> MASWSHPQFEKGASTSLYKKAGLMDSQRSTLVHWFRKGLRLHDNPALSHIFTAANAAPGRYFVRPIFILDPGILDWMQVGANRWRFLQQTLEDLDNQLRKLNSRLFVVRGKPAEVFPRIFKSWRVEMLTFETDIEPYSVTRDAAVQKLAKAEGVRVETHCSHTIYNPELVIAKNLGKAPITYQKFLGIVEQLKVPKVLGVPEKLKNMPTPPKDEVEQKDSAAYDCPTMKQLVKRPEELGPNKFPGGETEALRRMEESLKDEIWVARFEKPNTAPNSLEPSTTVLSPYLKFGCLSARLFNQKLKEIIKRQPKHSQPPVSLIGQLMWREFYYTVAAAEPNFDRMLGNVYCMQIPWQEHPDHLEAWTHGRTGYPFIDAIMRQLRQEGWIHHLARMAVACFLTRGDLWISWEEGQRVFEQLLLDQDWALNAGNWMWLSASAFFHQYFRVYSPVAFGKKTDPQGHYIRKYVPE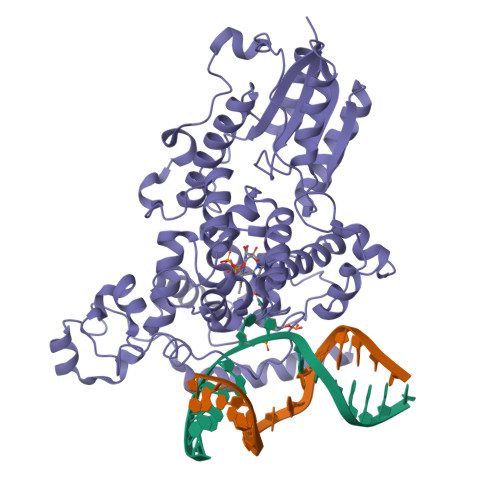LSKYPAGCIYEPWKASLVDQRAYGCVLGTDYPHRIVKHEVVHKENIKRMGAAYKVNREVRTGKEEESSFEEKSET>AFTACEKQTIGKIAQVLAKSPEAYGAECLARLFVTHPGSKSYFEYKDYSAAGAKVQVHGGKVIRAVVKAAEHVDDLHSHLETLALTHGKKLLVDPQNFPMLSECIIVTLATHLTEFSPDTHCAVDKLLSAICQELSSRYR[2x];>VHWTQEERDEISKTFQGTDMKTVVTQALDRMFKVYPWTNRYFQKRTDFRSSIHAGIVVGALQDAVKHMDDVKTLFKDLSKKHADDLHVD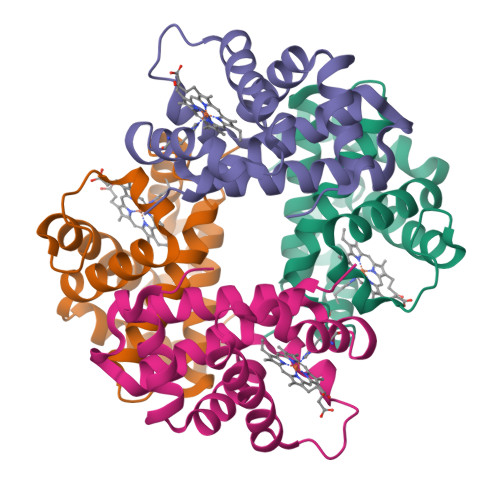PGSFHLLTDCIIVELAYLRKDCFTPHIQGIWDKFFEVVIDAISKQYH[2x]>[2x]MSNKYRVRKNVLHLTDTEKRDFVRTVLILKEKGIYDRYIAWHGAAGKFHTPPGSDRNAAHMSSAFLPWHREYLLRFERDLQSINPEVTLPYWEWETDAQMQDPSQSQIWSADFMGGNGNPIKD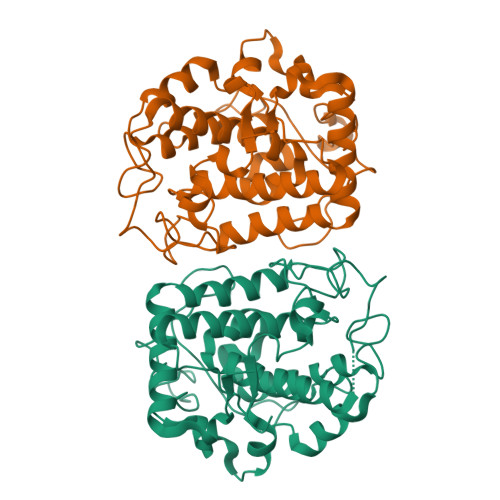FIVDTGPFAAGRWTTIDEQGNPSGGLKRNFGATKEAPTLPTRDDVLNALKITQYDTPPWDMTSQNSFRNQLEGFINGPQLHNRVHRWVGGQMGVVPTAPNDPVYFLHHANVDRIWAVWQIIHRNQNYQPMKNGPFGQNFRDPMYPWNTTPEDVMNHRKLGYVYDIELRKSKRSSHHHHHH> SRPTKFQDKYYIPVDQYPDVNFVGLLLGPRGRTLRKLQEDSNCKIAIRGRGSVKEGKNASDLPPGAMNFEDPLHCLIMADSEDKMQKGIKVCQNIMIKAVTSP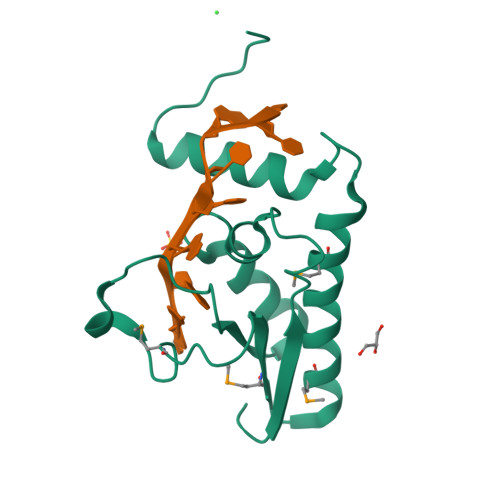EGQNDLKRGQLRELAELNGTLREDNR>[3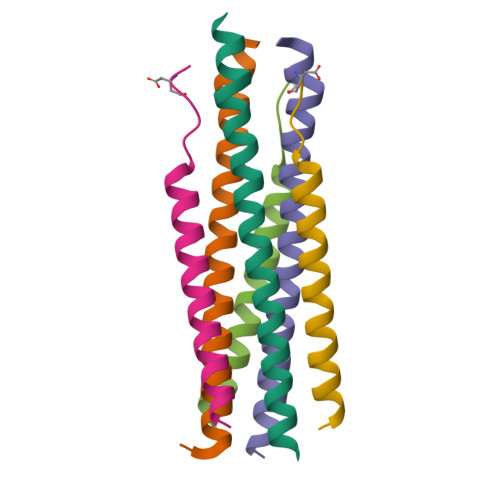x]XQARSDIEKLKEAIRDTNKAVQSVQSSIGNLIVAIKSVQDYVNKEIVPSIARX;>XVALDPIDISIVLNKIKSQLEESKEWIRRSNKILDSIX[3x]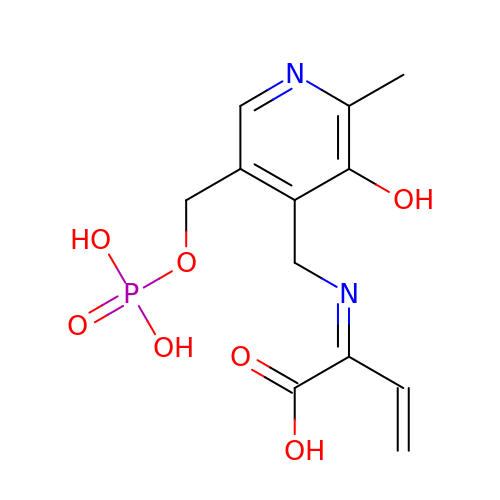(2E)-2-[({3-hydroxy-2-methyl-5-[(phosphonooxy)methyl]pyridin-4-yl}methyl)imino]but-3-enoic acid | C12 H15 N2 O7 P | ILCWREDNKMRIGC-GXDHUFHOSA-N>TEHLTLAFKIERPYDKVLKTISKKNLKNYIKETFNFFKSGYMK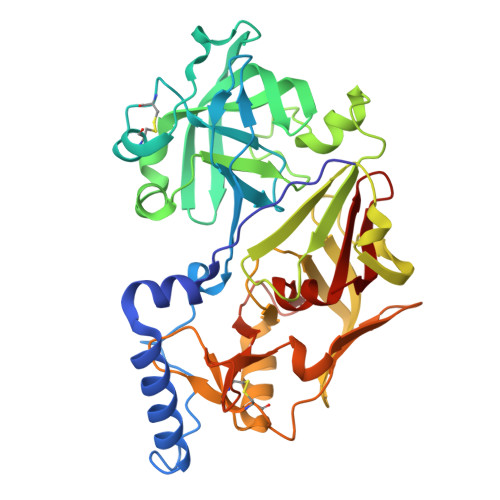QNYLGSENDVIELDDVANIMFYGEGEVGDNHQKFMLIFDTGSANLWVPSKKCNSSGCSIKNLYDSSKSKSYEKDGTKVDITYGSGTVKGFFSKDLVTLGHLSMPYKFIEVTDTDDLEPIYSSVEFDGILGLGWKDLSIGSIDPIVVELKNQNKIDNALFTFYLPVHDVHAGYLTIGGIEEKFYEGNITYEKLNHDLYWQIDLDVHFGKQTMEKANVIVDSGTTTITAPSEFLNKFFANLNVIKVPFLPFYVTTCDNKEMPTLEFKSANNTYTLEPEYYMNPILEVDDTLCMITMLPVDIDSNTFILGDPFMRKYFTVFDYDKESVGFAIAKN[2x]> MTPPKAEKRPYPITTHGDTRVDDYYWLRDDERTDPQVLDYLQAENAFTDAALKPQQALRETLYEEMVARIPQQEHSVPYVRHGYRYQTRFEPGNEYAIYVRQPQAESEHWDTLIDGNQRAEQREFYTLGGLEVSPDNQKLAVAEDFLSRRQYDIRFKNLSDDSWTDEVLENTSGSFEWANDSATVYYVRKHAKTLLPYQVYRHVVGTDPQLDELIYEEQDDTFYVGLEKTTSDRFILIHLSSTTTSEILLLDADRADSTPQMFVPRRKDHEYGIDHYHQHFYIRSNKDGKNFGLYQSEQADEAQWQTLIAPRIEVMLEGFSLFRDWLVVEERSEGLTQLRQIHWQSGEVKRIAFDDPTYTTWLAYNPEPETELLRYGYSSMTTPTTLYELNLDSDERVMLKQQEVKNFTPENYRSERVWVKARDGVEVPVSLVYRHDSFARGTNPLMVYGYGSYGSSMDPAFSASRLSLLDRGFVFVLAHIRGGGELGQLWYEDGKLFKKQNTFNDFIDVTEALIAQGYGDAKRVFAMGGSAGGLLMGAVINQAPELFNGIVAQVPFVDVVTTMLDESIPLTTGEYDEWGNPNQQAYYDYILQYSPYDQVKAQDYPHMLVTTGLHDSQVQYWEPAKWVAKL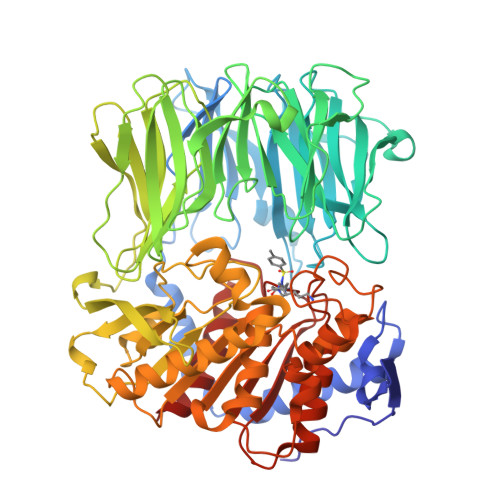RELKTDDRQLLLYTDMDSGHGGKSGRFKAYEDIALEYAFILALAE> DVMTKEEQIFLLHRAQAQCE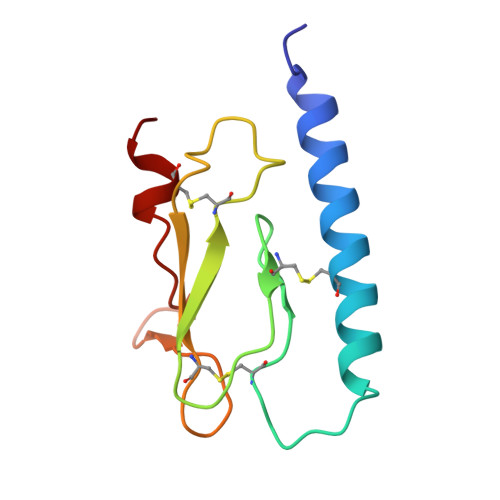KRLKEVLQRPAGRPCLPEWDHILCWPLGAPGEVVAVPCPDYIYDFNHKGHAYRRCDRNGSWELVPGHNRTWANYSECVKFL>CCACTAG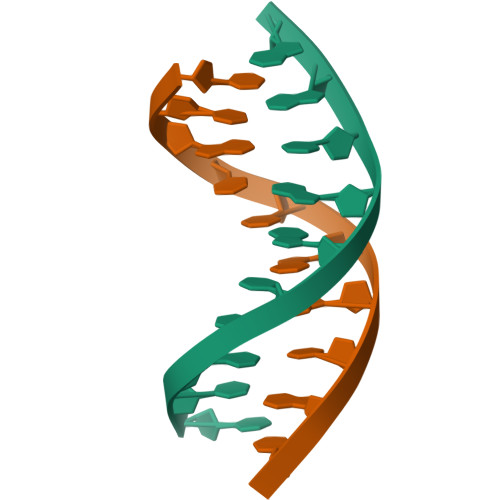TGG[2x]BREX (Bacteriophage Exclusion) systems, identified through shared identity with Pgl (Phage Growth Limitation) systems, are a widespread, highly diverse group of phage defence systems found throughout bacteria and archaea. The varied BREX Types harbour multiple protein subunits (between four and eight) and all encode a conserved putative phosphatase, PglZ, and an equally conserved, putative ATPase, BrxC. In this study, we identified a stable BREX sub-complex of PglZ:BrxB, generated and validated a structural model of that protein complex, and assessed the biochemical activity of PglZ from BREX, revealing it to be a metal-dependent nuclease. PglZ can cleave cyclic oligonucleotides, linear oligonucleotides, plasmid DNA and both non-modified and modified linear phage genomes.

Large scale co-expression and co-purification of His-SUMO-BrxB and PglZ yielded a clean sample of native PglZ:BrxB sub-complexes. The Salmonella PglZ:BrxB sub-complexes were used to perform structural studies through negative stain transmission electron microscopy, followed by cryo-EM. The final model displayed a GSFSC resolution of 4.45 Å, but the features of the resulting map, while clearly indicating the presence of a protein volume and dimensions consistent with a PglZ:BrxB complex, did not provide clearly defined features corresponding to individual secondary structural elements, likely caused by the influence of very strong preferred orientation of the particles, with a corresponding cFAR value reported by orientation diagnostics in CryoSPARC of 0.04. BrxB is itself predicted with high confidence to form a globular protein fold, and further predicted to interact with the N-terminal domain (residues 1–96) of PglZ. Examination of the model using EMBL PISA identified Salmonella BrxB residues R49, N135 and W137, and PglZ residues K58, E62 and D88, as forming the core of the predicted protein–protein interface (inset). The remainder of the PglZ protein is predicted to assume an ‘S’ shape, similar to observed particles from the EM analyses with a central domain (residues 98–292) and a large C-terminal domain (residues 304–748) that contains the metal-binding site identified within PorX, and a final extension including a seven sheet β-barrel (residues 749–867). However, the orientations of those two modelled regions, relative to one another, differ significantly when comparing the same independent AlphaFold3 predictions, consistent with a possible flexible hinge point in the protein backbone located between residues 96 and 99 of PglZ. Collectively, our mutational analysis of the PglZ:BrxB interface supports our hybrid cryo-EM and AlphaFold3 model. Alternatively, and due to the observed data in Salmonella and E. coli, we postulate that the role of BrxB might be as a scaffold protein, participating within and allowing connections between multiple BREX components within higher order complexes.

> IDPVLEYRLSQVQSRISEERFLKNNGSGNEIGFWIFDYPAQNELQVREHLKYLLRNLEKDHKFAHLNIFQIIVDMLTERGLFDRVCQQEVKVGTEALKKQLVGLLNQKKIADYIAKKVDLQNQEFVILTGMGNAWPLVRGHELMSALQDVMGFTPLLMFYPGTYSGHDLSPLAGIDSRNYYRAFRLVPESGPAATLNPR;> MTLQNQEFIAGLKAKFAEHRIVFWHDPDKRFLEELDNLELENVTLLDMTDQSQLAVKKRIEIDEPEQQFLLWFPHDAPPKEFDWLLDIRLYSTEFHADFAAITLNTLGIPQLGLREHIQRRKAFFSTKRLSALKGLVTEQENEASLDKKMVAVIAGVKTAKTEEILFSLITQYVNQQKDDDSDLENTLAMLKRHDLEGVLWDILNQEMGYQAEHPTLENLILKLFCTDLSAQADPQKREWLEKNVLATPSGRASALAFMVTWRADRRYKEAYDYCAQQMQDALRPEDQYRLSSPYDLHECETTLSIEQTIIHALVTQLLEESTTLDREAFKKLLSERQSKYWCQTRQEYCAIYDALRQAERLLNLRNRHIDGFHYQDSATFWKAYCEELFRFDQAYRLFNEYALLVHSKGAMILKSLDDYIEALYSNWYLAELSRSWNKVLETENRMQEWRIAGVPRQQNFYNEVVKPQFNNPQIKRVFVIISDALRYEVAEELGNQINTEKRFTAELRSQLGVLPSYTQLGMAALLPHDEICYQPGSGDIVYADGLSTSGTPNRDTILKKYKGMAVKSDDLLKWKNQQGRDLIRDYEVVYIWHNTIDAMGDSASTEEKTFEACRNAVVELKDLVTRVINRLHGTRIIVTADHGFLFQQQPLSGQDKTTLQIKPDNTIKNHKRFIIGHQLPADDFCWKGKVADTAGVSDNSEFLIPKGIQRFHFSGGARFVHGGAMLQEVCVPVLQVKALQKTAAEKQPQRRPVDIVKHHPLIKLVNNIDKVSLLQTHPVGELYEPRTLNIFIVDNANNVVSGKERICFDSDNNTMEKRVRDVTLKLIGANFNRRNEYWLILEDAQTETGYQKYPVIIDLAFQDDFFKETAAAKFERQHMDSSTSAA> QAADDRQLLIRIKRVWRDPPVLAAWNGSGDHCTWPYVTCDASGRVTSLSLANTGVAGPFPDAIGGLSGLTSLDLSGNYLDGELPADIGRALGKNLTSLMLNGNYFNGTIPTSLSRLKNLQSLALDNNFLAGTIPAELGDLTGLQMLTLANNSFSVGVLPASFKNLTQLKTFWAAICNLTGDFPSYVAEMRELEVLDLSVNALTGSIPPAIWNLAKLQTMALFANNFTGGVVVADGAFSAVNLVMIDLSSNHRLSGPIPEAFGHLPNLETLNLYFNNFSGEIPASIGRLPSLVTLSLFRNRLTGRLPPDLGKNSSAGLMYIDVDDNEISGAIPEGLCANGKFQSLIARNNRLNGSIPAGLASCATLNNLMLGNNQLSGEVPEALWTVPQLEYVLLRNNRLSGSLPVKMFINLSTLHIENNQFGGNIPAAAVGLREFIAGNNNFSGEMPASLGKGMPLLQAMNLSGNQLFGGIPSSVAKLRLLTQLDLSRNQLAGEIPAELGAMRVLSALDLSSNKLS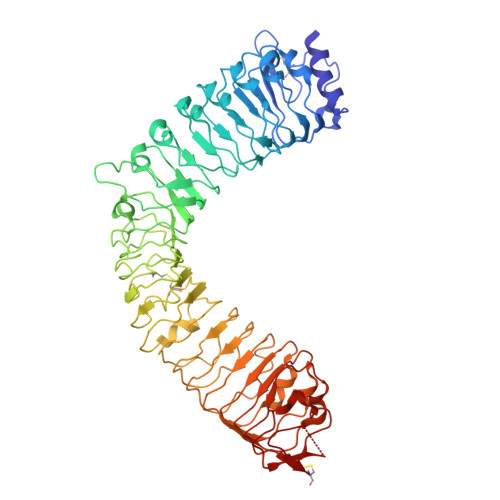GYIPPPLAGLPLTFLNLSSNQLDGQVPAGLATAAYDRSFLGNPGLCHAGLGPRYLTGVRSCAAGS>GPLGSHMSTESNDGVSETLLAWRHIDFWTSEHNPDLNATLSDPCTQNDITHAEEDLEVSFPNPVKASFKIHDGQEDLESMTGTSGLFYGFQLMTLDQVVAMTQAWRNVAKNLNKRSQQGLSHVTSTGDSSSMERLNGNKFKLPNIPDQKSIPPNAVQPVYAHPAWIPLITDNAGNHIGVDLAPGPNGKYAQIITFGRDFDTKFVIAENWGEFLLSFANDLEAGNWYLVDDNDDYFSGDGELVFRDKKSNGPIQDYFEVLKRRTWI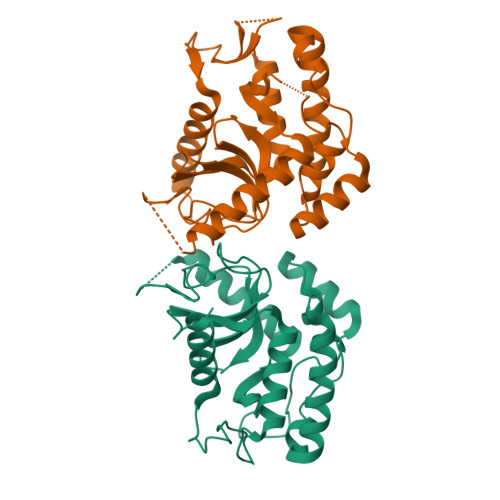KYQLERPHRD[2x]> GHMSHLADVSPPTACRVCGGGVQEFLDLGRQPLSDRFRKPDELDDEFTYRLAVGRCDSCEMVQLTEEVPRDLMFHEVYPYHSSGSSVMREHFAMLARDFLATELTGPDPFIVEIGCNDGIMLRTIQEAGVRHLGFEPSSGVAAKAREKGIRVRTDFFEKATADDVRRTEGPANVIYAANTLCNIPYVQSVLEGVDALLAPDGVFVFEDPYLGDIVAKTSFDQIYDQHFFLFSATSVQGMAQRCGFELVDVQRLPVHGGEVRYTLARQGSRTPSAAVAQLLAAEREQELSDMATLRAFAG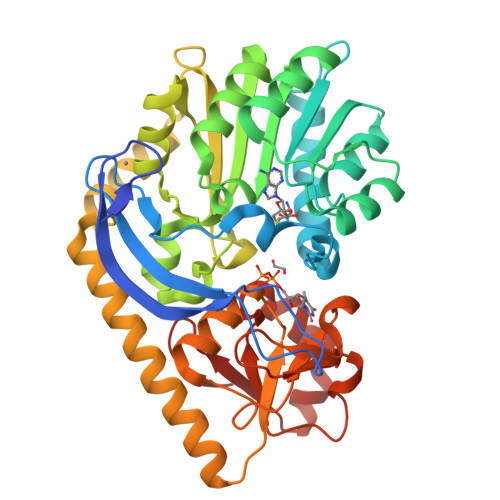NVVKIRDELTALLHRLRAEGRSVVGYGATAKSATVTNFCGIGPDLVHSVYDTTPDKQNRLTPGAHIPVRPASAFSDPYPDYALLFAWNHAEEIMAKEQEFHQAGGRWILYVPEVHIR>[2x]GPHMARKFFVGGNWKCNGTAEEVKKIVNTLNEAQVPSQDVVEVVVSPPYVFLPLVKSTLRSDFFVAAQNCWVKKGGAFTGEVSAEMLVNLDIPWVILGHSERRAILNESSEFVGDKVAYALAQGLKVIACVGETLEEREAGSTMDVVAAQTKAIADRVTNWSNVVIAYEPVWAIGTGKVASPAQAQEVHDELRKWLAKNVSA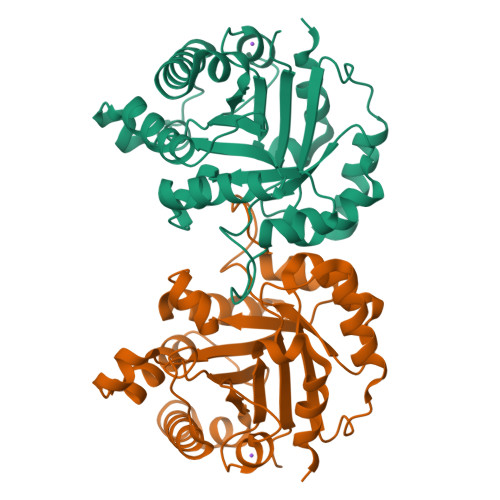DVAATTRIIYGGSVNGGNKKELGGQADVDGFLVGGASLKPEFIDIIKAAEVKKSA>[4x]MTHHYPTDDIKIKEVKELLPPIAHLYELPISKEASGLVHRTRQEISDLVHGRDKRLLVIIGPCSIHDPKAALEYAERLLKLRKQYENELLIVMRVYFEKPRTTVGWKGLINDPHLDGTFDINFGLRQARSLLLSLNNMGMPASTEFLDMITPQYYADLISWGAIGARTTESQVHRELASGLSCPVGFKNGTDGNLKIAID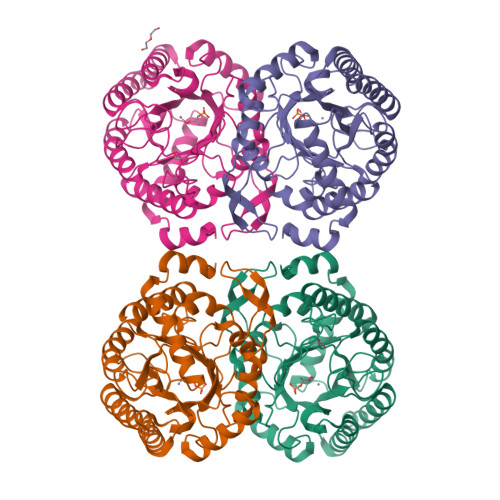AIGAASHSHHFLSVTKAGHSAIAHTGGNPDCHVILRGGKEPNYDAEHVSEAAEQLRAAGVTDKLMIDCSHANSRKDYTRQMEVAQDIAAQLEQDGGNIMGVMVESHLVEGRQDKPEVYGKSITDACIGWGATEELLALLAGANKKRMARAS>SNASKMSDVKCTSVVLLSVLQQLRVESSSKLWAQCVQLHNDILLAKDTTEAFEKMVSLLSVLLSMQGAVDINKLCEEMLDNRATLQ[2x];>EDKRAKVTSAMQTMLFTMLRKLDNDALNNIINNARDGCVPLNIIPLTTAAKLMVVIPDYNTYKNTCDGTTFTYASALWEIQQVVDADSKIVQLSEISMDNSPNLAWPLIVTALRANSAVKLQ[2x]

SARS-CoV-2 RdRp, also referred to as nonstructural protein 12 (Nsp12), is the catalytic center of the macromolecular complex frequently referred to as the replication transcription complex (RTC). The RTC is essential for virus replication because it makes copies of genomic and subgenomic RNAs and polymerizes antisense RNA. In SARS-CoV-2, besides RdRp (Nsp12), the RTC involves nonstructural proteins Nsp7, Nsp8, and others. Nsp12 is the largest component of the complex, and Nsp7 and Nsp8 are considered cofactors.

We have solved a 1.5 Å x-ray macromolecular crystal structure of the complex between Nsp7 and Nsp8. Below, the description of the Nsp7/8 structure is based on the 1.5 Å structure Nsp7/8C, unless otherwise mentioned. Nsp7 has three consecutive α-helices (α1, α2, and α3) forming a three-helical coiled-coil bundle and the C-terminal loop (residues 62–70) that in some structures is followed by a short, not well-defined helix (residues 68–72). The conformation of Nsp8 has previously been described to resemble a golf club (Fig. 1 A; (9)). The interface between Nsp7 and Nsp8 is made through hydrophobic contacts between six bundled helices. The helices involved are the two N-terminal helices (α1 and α2) from Nsp8 and four helices from Nsp7. The dimer interface area is 2834 Å2 with 72% hydrophobic contacts. Importantly, a symmetrically related interchain disulfide bond is also found between Cys8 of Nsp7 and its symmetry mate.In this study, we used solution NMR to investigate the conformational states of small-molecule inhibitors bound to LpxC, an essential metalloamidase that catalyses the deacetylation of UDP-(3-O-acyl)-N-acetylglucosamine during the biosynthesis of lipid A in Gram-negative bacteria. We chose Aquifex aeolicus LpxC (AaLpxC) in the lipid A biosynthetic pathway for structural and dynamics investigation due to its exceptional thermostability, which has enabled both NMR measurements and crystallographic studies (for example, refs 13, 14, 15, 16). Pseudomonas aeruginosa LpxC (PaLpxC) was exploited when co-crystal structures of the desired AaLpxC-inhibitor complexes could not be obtained. We show that these enzyme-bound inhibitors dynamically access alternative, minor conformations in solution in addition to the ligand state observed in the crystal structure.

Replacing the tail group of CHIR-090 with a substituted biphenyl diacetylene group generated LPC-011 with improved antibiotic activity due to minimization of vdW clashes with the substrate-binding passage. To provide a direct comparison with solution NMR investigations, we determined the crystal structure of AaLpxC in complex with LPC-011. This structure reveals a single conformation of the threonyl-hydroxamate head group in the active site, with the threonyl Cγ2 methyl group packing against an invariant phenylalanine residue (F180 in AaLpxC) and the Oγ1 hydroxyl group forming a hydrogen bond with the catalytically important lysine residue (K227 in AaLpxC). The threonyl side chain of the inhibitor features a trans configuration with a χ1 angle of 180°, a rotameric state that is less energetically favourable (7% population of all threonine side chains in proteins) compared with the alternative rotameric states of gauche- (χ1=−60°) and gauche+ (χ1=60°) collectively accounting for 92% of the observed threonine side-chain conformations. Since the observed ligand conformation in the crystal structure represents an unfavourable χ1 rotameric state of the threonyl head group, we investigated whether this group could access alternative ligand conformations in solution. Measurements of LPC-011 yielded a 3JNCγ2 coupling of 0.58±0.05 Hz and a 3JC'Cγ2 coupling of 0.77±0.04 Hz, corresponding to a predominant trans χ1 configuration with a population of 0.65±0.03. Such an observation is consistent with the ligand conformation in the AaLpxC/LPC-011 crystal structure. However, the measurements also revealed that the threonyl side chain of LPC-011 can readily access alternative, minor conformational states with a population of 0.23±0.03 for the gauche- χ1 conformation and a population of 0.12±0.01 for the gauche+ χ1 conformation.

>MGLEKTVKEKLSFEGVGIHTGEYSKLIIHPEKEGTGIRFFKNGVYIPARHEFVVHTNHSTDLGFKGQRIKTVEHILSVLHLLEITNVTIEVIGNEIPILDGSGWEFYEAIRKNILNQNREIDYFVVEEPIIVEDEGRLIKAEPSDTLEVTYEGEFKNFLGRQKFTFVEGNEEEIVLARTFAFDWEIEHIKKVGLGKGGSLKNTLVLGKDKVYNPEGLRYENEPVRHKVFDLIGDLYLLGSPVKGKFYSFRGGHSLNVKLVKELAKKQKLTRDLP[2x]> GRCYKSKPPICF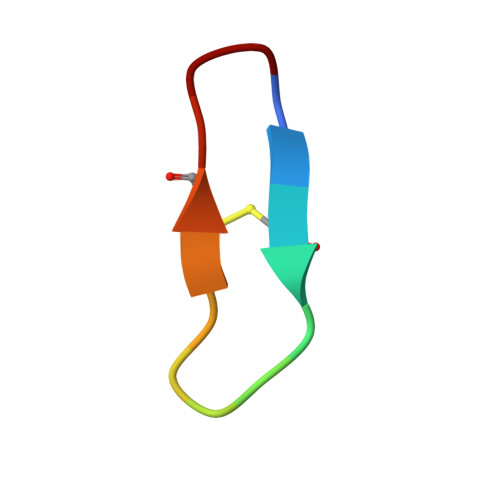PD> MNEQLNHLYGLPSHAIEALKCVFKEYSQIDNAILYGSRAKGTYHQGSDIDLCLTGNLLGITELLAIENKID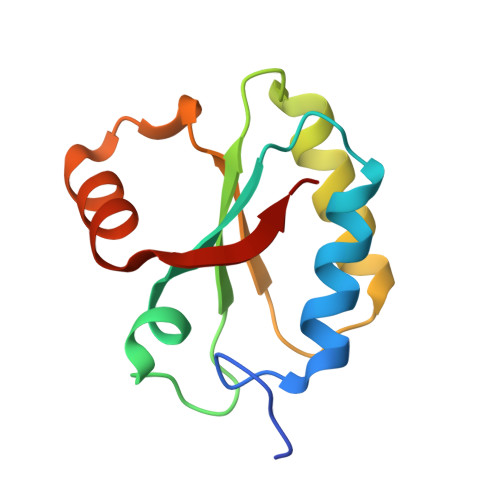DLLLPWKVDISLKHTIDNPDLLEHIERAGILFYTKES>ASGLFTIPDGDFFSTARAIVASNAVATNEDLSKIEAIWKDMKVPTDTMAQAAWDLVRHCADVGSSAQTEMIDTGPYSNGISRARLAAAIKEVCTLRQFCMKYAPVVWNWMLTNNSPPANWQAQGFKPEHKFAAFDFFNGVTNPAAIMPKEGLIRPPSEAEMNAAQTAAFVKITKARAQSNDFASLDAAVTRGRI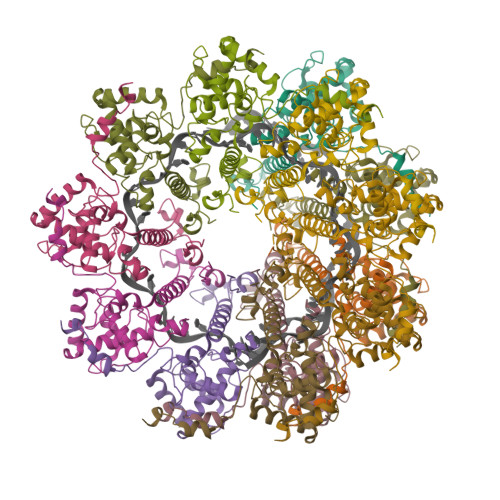TGTTTAEAVVTLPPP[13x]>GHMSLHPVSISLSSYGADLVRSRGQASFLPLLAMAGAQRVELREELFAGPPDTEALTAAIQLQG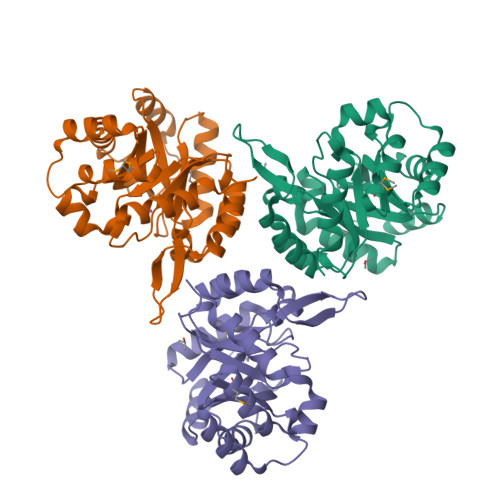LECVFSSPLELWREDGQLNPELEPTLRRAEACGAGWLKVSLGLLPEQPDLAALGRRLARHGLQLLVENDQTPQGGRIEVLERFFRLAERQQLDLAMTFDIGNWRWQEQAADEAALRLGRYVGYVHCKAVIRNRDGKLVAVPPSAADLQYWQRLLQHFPEGVARAIEYPLQGDDLLSLSRRHIAALARLGQPQEERQHGGS[3x]> MASGLVASNLNLKPGESLRVRGEVAPDAKSFVLNLGKDSNNLCLHFNPRFNAHGDANTIVSNSKDGGAWGTEQREAVFPFQPGSVAEVSITFDQANLTVKLPDGYEFKFPNRLNLEAINYMAADGDFKIKSVAFDGSSASGLVASNLNLKPGESLRVRGEVAPDAKSFVLNLGKDSNNLCLHFNPRFNAHGDANTIVSNSKDGGAWGTEQREAVFPFQPGSVAEVSITFDQANLTVKLPDGYEFKFPNRLNLEAINYM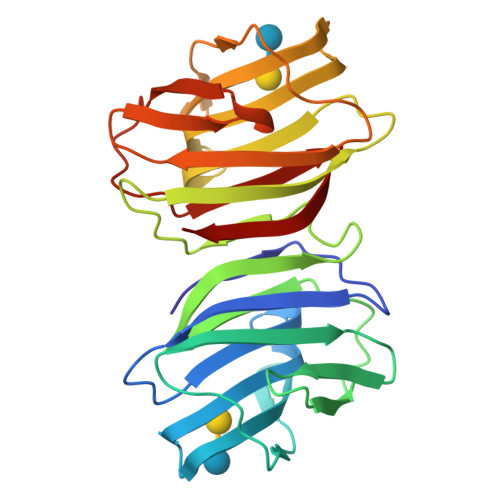AADGDFKIKSVAFD>[2x]GEIQWMRPSKEVGYPIINAPSKTKLEPSAFHYVFEGVKEPAVLTKNDPRLKTDFEEAIFSKYVGNKITEVDEYMKEAVDHYAGQLMSLDINTEQMCLEDAMYGTDGLEALDLSTSAGYPYVAMGKKKRDILNKQTRDTKEMQKLLDTYGINLPLVTYVKDELRSKTKVEQGKSRLIEASSLNDSVAMRMAFGNLYAAFHKNPGVITGSAVGCDPDLFWSKIPVLMEEKLFAFDYTGYDASLSPAWFEALKMVLEKIGFGDRVDYIDYLNHSHHLYKNKTYCVKGGMPSGASGTSIFNSMINNLIIRTLLLKTYKGIDLDHLKMIAYGDDVIASYPHEVDASLLAQSGKDYGLTMTPADKSATFETVTWENVTFLKRFFRADEKYPFLIHPVMPMKEIHESIRWTKDPRNTQDHVRSLCLLAWHNGEEEYNKFLAKIRSVPIGRALDLPEYSTLYRRWLDSFGSSSHHHHHH

The replication of positive-strand RNA viruses relies on virally encoded RNA-dependent RNA polymerases (RdRPs) that are capable of rapid and processive synthesis of the 7–14 kilobase viral genomes. To examine this in further detail and to validate the polymerase–RNA interactions seen in the initial poliovirus EC structures, we here present nine new coxsackievirus, rhinovirus, and poliovirus elongation complex structures at resolutions ranging from 2.1 to 2.9 Å. All the complexes feature an upstream RNA duplex that is pinched between the pinky finger and thumb domains such that the RNA exit channel is opened by ≈4 Å as compared to the polymerase alone structures. All of the complexes show the open conformation for the active site wherein the β-strands of motifs A and C are not hydrogen bonded together to fully form the RMM-fold that is commonly utilized by polymerase active sites.

Last, we further extended the length of the RNA duplex to 30 base pairs with a longer (GA)3 locking sequence in the r5 RNA and were able to obtain a third structure of the PV polymerase EC at 2.9 Å resolution (PV_r5). A CTP soak of the poliovirus 3Dpol PV_r5 crystal resulted in two nucleotide incorporation events and two translocation steps, giving a final state 1 structure that is essentially identical to the starting point, only with sequence variation in the RNA strands. The RNA-mediated lattice contacts of this crystal form allowed for significant twisting of one EC relative to the other within the dumbbell pair, but the structure within each EC was essentially unchanged. The nearly opposite behavior is seen in the PV_r5 lattice, where one and two translocation steps in each EC leads to a systematic movement of one polymerase relative to the other that is accommodated by twisting and sliding movements at the RNA-RNA junction point. In contrast, the PV_r5 structure shows significant rotations of one EC relative to the other and repacking of the RNA-RNA junction as the crystal lattice is reshaped to accommodate the longer upstream duplex regions. 2Fo–Fc maps contoured at 2.0 σ are shown for the PV_r5 structures where addition of 2′-dCTP results in one incorporation and translocation event while CTP addition results in two cycles of incorporation and translocation. Despite this common lattice organization, the different dumbbell pairs and their RNA-RNA junctions displayed a multitude of geometries in the different crystal forms; for example, the junctions in the PV EC structures range from near perfect coaxial stacking to highly disordered structures that could not be fully modeled into the electron density maps. A comparison of all the RNA-RNA junctions, shown in Figure 3, reveals geometries ranging from fairly straight and essentially canonical coaxial stacking (PV_r3, CV_r2) to slightly offset helical ends (PV_r1) to highly distorted geometries with frayed ends (PV_r5+2).> QDYKDDDDKHHHHHHHHHHENLYFQSHVLFIFPRTSGVKCPFPSRPDNGFVNYPAKPTLYYKDKATFGCHDGY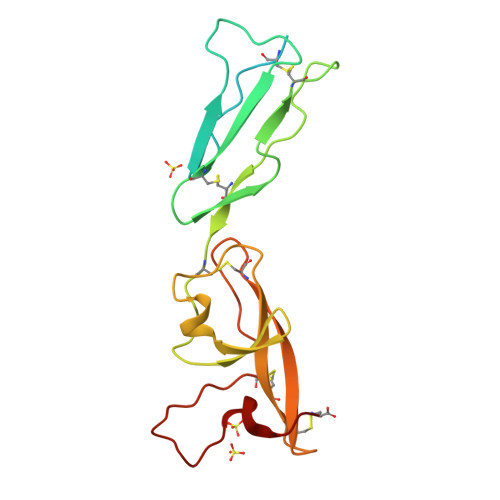SLDGPEEIECTKLGNWSAMPSCKASCKVPVKKATVVYQGERVKIQEKFKNGMLHGDKVSFFCKNKEKKCSYTEDAQCIDGTIEVPKCFKEHSSLAFWKTDASDVKPC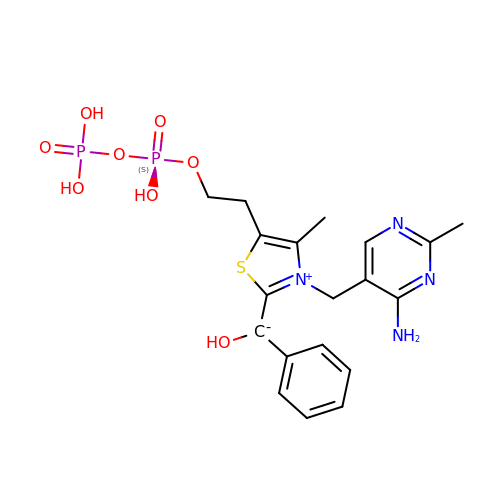C2-1-HYDROXYPHENYL-THIAMIN DIPHOSPHATE | C19 H24 N4 O8 P2 S | ZOLUTNQCUQSPSG-UHFFFAOYSA-N>[55x]MGLFDRIKRVVSSNLNDLVNKAEDPEKMLEQAILEMQEDLVQLRQGVAQAIAAQKRSEKQYNDAQNEINKWQRNAQLALQKGDENLARQALERKKTYTDTSAALKASLDTQSTQVETLKRNLIQLESKISEAKTKKEMLKARITTAKAQEQLQGMVRGMNTSSAMSAFERMEEKVLMQESRAQALGELAGADLETQFAQLEGGSDVDDELAALKAQMLPPATPVTQAQLPPQQETTPAKSNEVVDAELDSLRKQLDQL

Proteins that perform these functions include Vipp1/IM30 in photosynthetic plastids, PspA in bacteria, and ESCRT-III in eukaryotes. Here, using a combination of evolutionary and structural analyses, we show that these protein families are homologous and share a common ancient evolutionary origin that likely predates the last universal common ancestor. This homology is evident in cryo-electron microscopy structures of Vipp1 rings from the cyanobacterium Nostoc punctiforme presented over a range of symmetries. Rings have an inner lumen that is able to bind and deform membranes.

Reconstructions were also generated for the other six symmetries and complete ring models built. To test whether the dome-shaped curvature observed in Vipp1 rings depends on a combination of inter-rung contacts and geometric constraints, as suggested by these data, an idealized elastic-network model of the Vipp1C11 ring was constructed. The model rings formed Vipp1-like dome-shaped curvature with helix α5 rotation (Δϕi) increasing with rung distance from the ring equator. Strikingly, the cumulative helix α5 rotation (Δϕ) between all rung interfaces plateaued near 40°, indicating a strict geometrical bending limit. Remarkably, this maximal rotation within the simulated stacks closely matched the measured experimental Δϕ in Vipp1C11, as well as the cumulative ∼40° helix α5 rotations observed for Vipp1C14. Thus, the simulations suggest a simple self-regulatory mechanism for limiting ring stack size where stress from inter-rung rotation builds up until the formation of Interfaces 1 and 3 is no longer favorable beyond a geometrical limit of ∼40°, after which further stacking is impeded. When membrane was modeled into the Vipp1C11–C17 structures as a 4-nm bilayer, sequential constriction was observed with the membrane lumen reaching ∼3 nm within Vipp1C11. This is close to the biophysical limit required to induce membrane fusion/fission (Chernomordik et al., 1995; Kozlovsky and Kozlov, 2003).> ADNLAEFHVQNQECDSCHTPDGELSNDSLTYENTQCVSCHGTLAEVAETTKHEHYNAHASHFPGEVACTSCHSAHEKSMVYCDSCHSFDFNMPYAKKWLRDEPTIAELAKDKSERQAALASAPHDTVDVVVVGSGGAGFSAAISATDSGAKVILIEKEPVIGGNAKLAAGGMNAAWTDQQKAKKITDSPELMFEDTMKGGQNINDPALVKVLSSHSKDSVDWMTAMGADLTDVGMMGGASVNRAHRPTGGAGVGAHVVQVLYDNAVKRNIDLRMNTRGIEVLKDDKGTVKGILVKGMYKGYYWVKADAVILATGGFAKNNERVAKLDPSLKGFISTNQPGAVGDGLDVAENAGGALKDMQYIQAAPTLSVKGGVMVTEAVRGNGAILVNREGKRFVNEITTRDKASAAILAQTGKSAYLIFDDSVRKSLSKIDKYIGLGVAPTADSLVKLGKMEGIDGKALTETVARYNSLVSSGKDTDFERPNLPRALNEGNYYAIEVTPGVHHTM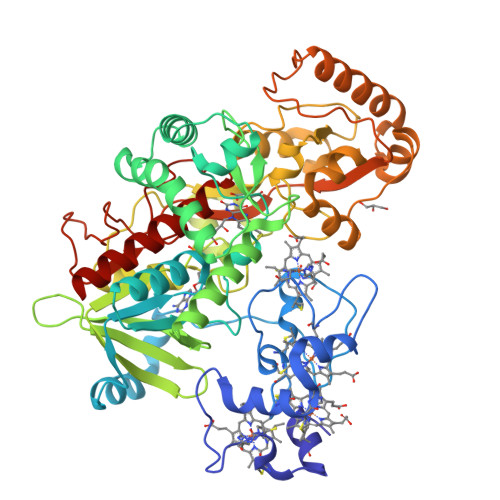GGVMIDTKAEVMNAKKQVIPGLYGAGEVTGGVHGANRLGGNAISDIITFGRLAGEEAAKYSKKN(2E)-1-[(1S)-1-benzylphthalazin-2(1H)-yl]-3-{5-[(2,4-diaminopyrimidin-5-yl)methyl]-2,3-dimethoxyphenyl}prop-2-en-1-one | C31 H32 N6 O3 | 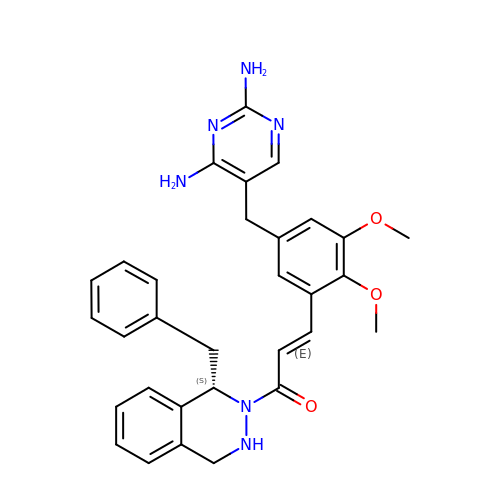OSCKDSROOCELQQ-JYSHFMIGSA-N> MMEGKEYIILKNPIANADNSLIEIFSYRCTHCYDHHKFNTMGKVKEKLPNLTYKFYPVSSMGDYGRQANEIFAFAAFKDGVNKIDPTDKNSLTHKVAKAYFNAYFKKKQRWENGK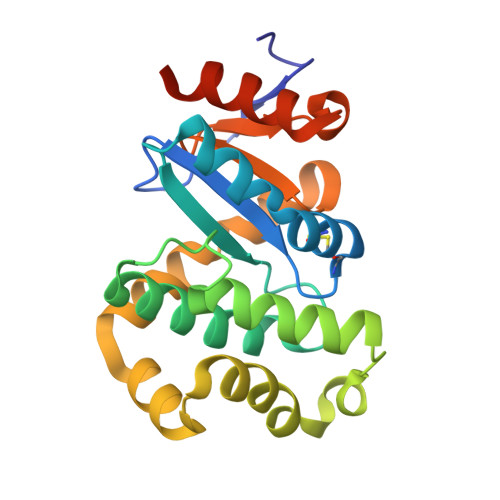NPEAFYSVGLKAMNVSKADLENFLKTPEAAELLKSYEIANPISQNYGTPAFVVNGKYQIIPSAINSPEALIEITKELSKQKLEHHHHHH> STAKAPTLPASIFRAYDIRGVVGDTLTAETAYWIGRAIGSESLARGEPCVAVGRDGRLSGPELVKQLIQGLVDCGCQVSDVGMVPTPVLYYAANVLEGKSGVMLTGDHNPPDYNGFKIVVAGETLANEQIQALRERIEKNDLASGVGSVEQVDILPRYFKQIRDDIAMAKPMKVVVDCGNGVAGVIAPQLIEALGCSVIPLYCEVDGNFPNHHPDPGKPENLKDLIAKVKAENADLGLAFDGDGDRVGVVTNTGTIIYPDRLLMLFAKDVVSRNP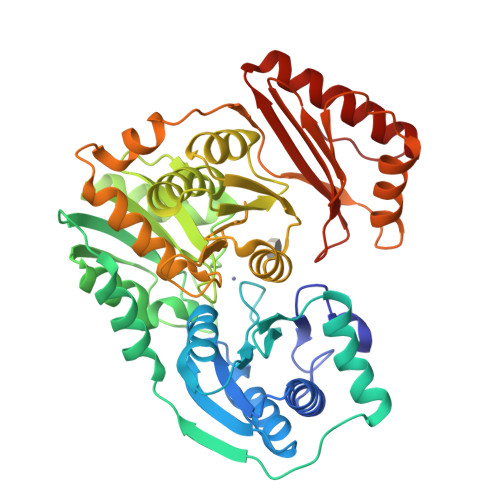GADIIFDVKCTRRLIALISGYGGRPVMWKTGHSLIKKKMKETGALLAGEMSGHVFFKERWFGFDDGIYSAARLLEILSQDQRDSEHVFSAFPSDISTPEINITVTEDSKFAIIEALQRDAQWGEGNITTLDGVRVDYPKGWGLVRASNTTPVLVLRFEADTEEELERIKTVFRNQLKAVDSSLPVPF> HHHHHHMSGENLYFQGASAAIVTDTGGVDDKSFNQSAWEGLQAWGKEHNLSKDNGFTYFQSTSEADYANNLQQAAGSYNLIFGVGFALNNAVKDA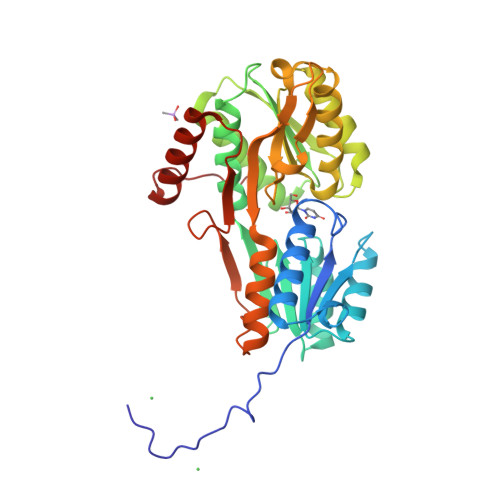AKEHTDLNYVLIDDVIKDQKNVASVTFADNESGYLAGVAAAKTTKTKQVGFVGGIESEVISRFEAGFKAGVASVDPSIKVQVDYAGSFGDAAKGKTIAAAQYAAGADIVYQVAGGTGAGVFAEAKSLNESRPENEKVWVIGVDRDQEAEGKYTSKDGKESNFVLVSTLKQVGTTVKDISNKAERGEFPGGQVIVYSLKDKGVDLAVTNLSEEGKKAVEDAKAKILDGSVKVPEK;>[2x]SSHHHHHHMSGENLYFQGASAAIVTDTGGVDDKSFNQSAWEGLQAWGKEHNLSKDNGFTYFQSTSEADYANNLQQAAGSYNLIFGVGFALNNAVKDAAKEHTDLNYVLIDDVIKDQKNVASVTFADNESGYLAGVAAAKTTKTKQVGFVGGIESEVISRFEAGFKAGVASVDPSIKVQVDYAGSFGDAAKGKTIAAAQYAAGADIVYQVAGGTGAGVFAEAKSLNESRPENEKVWVIGVDRDQEAEGKYTSKDGKESNFVLVSTLKQVGTTVKDISNKAERGEFPGGQVIVYSLKDKGVDLAVTNLSEEGKKAVEDAKAKILDGSVKVPEK;> SSHHHHHHMSGENLYFQGASAAIVTDTGGVDDKSFNQSAWEGLQAWGKEHNLSKDNGFTYFQSTSEADYANNLQQAAGSYNLIFGVGFALNNAVKDAAKEHTDLNYVLIDDVIKDQKNVASVTFADNESGYLAGVAAAKTTKTKQVGFVGGIESEVISRFEAGFKAGVASVDPSIKVQVDYAGSFGDAAKGKTIAAAQYAAGADIVYQVAGGTGAGVFAEAKSLNESRPENEKVWVIGVDRDQEAEGKYTSKDGKESNFVLVSTLKQVGTTVKDISNKAERGEFPGGQVIVYSLKDKGVDLAVTNLSEEGKKAVEDAKAKILDGSVKVPE> CPILWTRNGSHCYYFSMEKKDWNSSLKFCADKGSHLLTFPDNQGVKL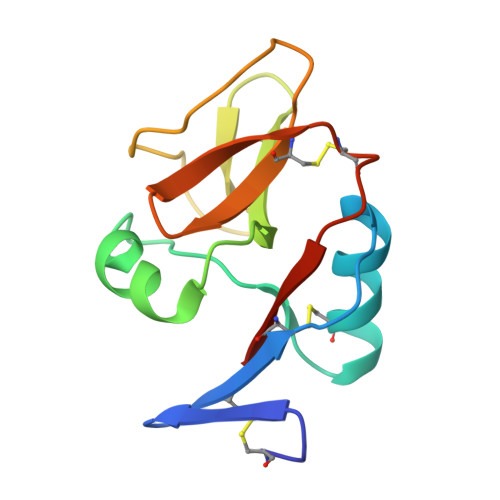FGEYLGQDFYWIGLRNIDGWRWEGGPALSLRILTNSLIQRCGAIHRNGLQASSCEVALQWICKKVLY P1,P6-Di(adenosine-5') hexaphosphate 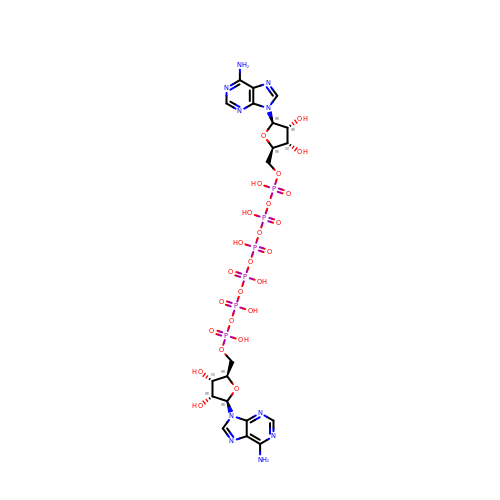| C20 H30 N10 O25 P6 | PZCFFCOJNXGTIM-XPWFQUROSA-N(3S)-3-hydroxy-D-aspartic acid | C4 H7 N O5 | 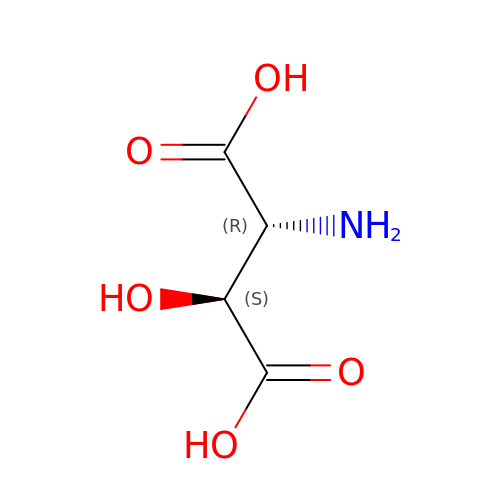YYLQUHNPNCGKJQ-NCGGTJAESA-N(2~{S},6~{S})-2-azanyl-6-[[(4~{R})-4-azanyl-5-oxidanyl-5-oxidanylidene-pentanoyl]amino]heptanedioic 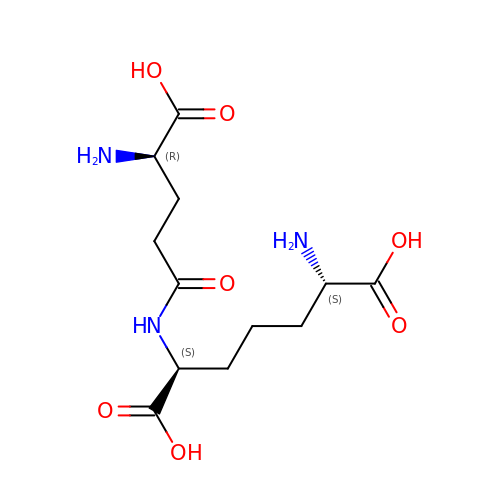acid | C12 H21 N3 O7 | QIFGMZZTJRULMA-RNJXMRFFSA-N> QSDLLVPKLTASVTDGAVGVTVDAPVSVTAADGVLAAVTMVNDNGRPVAGRLSPDGLRWSTTEQLGYNRRYTLNATALGLGGAATRQLTFQTSSPAHLTMPYVMPGDGEVVGVGEPVAIRFDENIADRGAAEKAIKITTNPPVEGAFYWLNNREVRWRPEHFWKPGTAVDVAVNTYGVDLGEGMFGEDNVQTHFTIGDEVIATADDNTKILTVRVNGEVVKSMPTSMGKDSTPTANGIYIVGSRYKHIIMDSSTYGVPVNSPNGYRTDVDWATQISYSGVFVHSAPWSVGAQGHTNTSHGCLNVSPSNAQWFYDHVKRGDIVEVVNTVGGTLPGIDGLGDWNIPWDQWRAGNAKA

The essential l,d-transpeptidase of Mycobacterium tuberculosis (LdtMt2) catalyses the formation of 3→3 cross-links in cell wall peptidoglycan and is a target for development of antituberculosis therapeutics. Whereas the d,d-transpeptidases catalyse the formation of 4→3 cross-links between peptidoglycan pentapeptide chains, the functionally related l,d-transpeptidases (Ldts) catalyse the formation of 3→3 cross-links between tetrapeptide chains. The Ldts, which do not manifest structural homology with the PBPs and likely originate from a different evolutionary precursor, share a common YkuD fold (named after the first identified member of this class), distinguished by a β-sandwich with two mixed β-sheets and one helix, and a set of four loops. The established substrate for LdtMt2 is the disaccharide tetrapeptide monomer 1 (GlcNAc-MurNAc-l-Ala-d-iGluNH2-m-DAPNH2-d-Ala).

Notably, however, when LdtMt2 and 3 were co-crystallised using a precipitation solution at pH 7.0, we observed additional electron density extending from the sidechain of the nucleophilic residue Cys354. The results are in agreement with formation of the dipeptide (d-iGluNH2-m-DAPNH2), covalently linked to LdtMt2 via a thioester with Cys354, apparently reflecting a key intermediate of the transpeptidase reaction with the donor peptide. In the LdtMt2-3 complex structure, the m-DAPNH2 residue sidechain protrudes into the outer cavity, while the d-iGluNH2 sidechain is located in the inner cavity, suggesting that the donor substrate enters from the inner cavity. Note that no electron density was observed corresponding to the l-Ala residue of 3, which has previously been suggested not to play a significant role in substrate binding. Additional electron density at the entrance of the outer cavity was observed, in which d-Ala, released during the formation of the thioester intermediate, could be modelled. The overall fold of the LdtMt2-3 complex strongly resembles that observed for unmodified LdtMt2 (PDB 6RLG27; main chain RMSD 0.65 Å). Notably, no conformational changes relative to unmodified LdtMt2 are observed in loop II, which encloses the active site (residues 300-323) and which has previously been observed to undergo conformational changes upon binding of various LdtMt2 inhibitors, and which has been proposed to undergo extensive conformational changes upon substrate binding. The thioester acyl group is located in the proposed oxyanion hole (the backbone NH groups of His352, Gly353 and Cys354) at respective distances of 3.8 Å, 3.3 Å and 2.3 Å, suggesting that, at least in the crystal structure obtained, no strong interactions are made with the backbone NH groups of His352. Polar interactions of m-DAPNH2 with His336 (3.0 Å), Asn356 (3.4 Å) and Thr320 (2.8 Å), as well as water-mediated polar interactions with His352 (3.3 Å to water, 3.4 Å to His352) are observed.Type III secretion systems (T3SS) allow the transport of protein substrates directly across the double membrane of Gram-negative bacteria. Proteomic analyses have identified the major components of the sorting platform for the Salmonella typhimurium SPI-1 injectisome: the AAA+ ATPase InvC, its regulator OrgB and the proteins SpaO and OrgA4. Here we show that a novel, heterotypic interaction between SPOA domains serves as a scaffold for sorting platform assembly in both injectisome and flagellar T3SS. Our structures suggest a partial model for the subtype-specific assembly of the T3SS sorting platforms: the heterotypic interaction between SPOA domains within a given T3SS subtype functions as an adaptor for ATPase and its regulator through interaction with the APAR peptide.

While SPOA1 alone was insoluble, constructs containing both SPOA1 and SPOA2 (residues 140–297) were stable and soluble. We hypothesized that SPOA2 interacts with and stabilizes SPOA1; consistent with this hypothesis, a SPOA1 construct (145–213) could be co-refolded with SPOA2. This complex crystalized, and its structure was determined to 2.9 Å resolution. SPOA1 and SPOA2 form a distinct, heterotypic SPOA–SPOA interaction with an overall topology similar to that of the SPOA2 homodimer. The SPOA1 backbone follows that of the prototypical SPOA fold, retaining the antiparallel beta-sheet floor and fingers-to-palm architecture. In both SPOA1,2 and the SPOA2 homodimer, interacting protomers each bury about 1,800 Å2 against their binding partner. SPOA1,2 and the SPOA2 homodimer superpose with 2.47 Å r.m.s.d. , and the conformation of SPOA2 in association with SPOA1 is grossly similar to that seen in the homodimer, superposing with an r.m.s.d. of 1.67 Å. The existence of heterotypic SPOA interactions provides a structural explanation for the observed ∼1:3 stoichiometry of SPOA1 to SPOA2 in SpaO homologues. We show here that the third SPOA2 can be stabilized by a SPOA1–SPOA2 interaction.

> GPVDPKMLRWPLRFVIGSSDTQRSLLGRIGIGDVLLIRTSRAEVYCYAKKLGHFNRVEGGIIVETLDIQHIEE;> GPVDVKLEFVLYRKNVTLAELEAMGQQQLLSLPTNAELNVEIMANGVLLGNGELVQMNDTLGVEIHEWLS> MVVNTIYIARHGYRSNWLPEGPYPDPLTGIDSDVPLAEHGVQQAKELAHYLLSLDNQPEAAFASPFYRCLETVQPIAKLLEIPVYLERGIGEWYRPDRKPVIPVPAGYEILSKFFPGVISQEWDSTLTPNEKGETEQEMYMRFKKFWPLFIERVEKEYPNVECILLVTHAASKIALGMSLLGYDNPRMSLNENGDKIRSGSCSLDKYEILKKSYDTIDETDDQTSFTYIPFSDRKWVLTMNGNTEFLSSGEEMNWNFDCVAEAGSDADIKKRQMTKKTSSPIPEADDQTEVETVYISVDIPSGNYKERTEIAKSAILQYSGLETDAPLFRIGNRLYEGSWERLVGTELAFPNAAHVHKK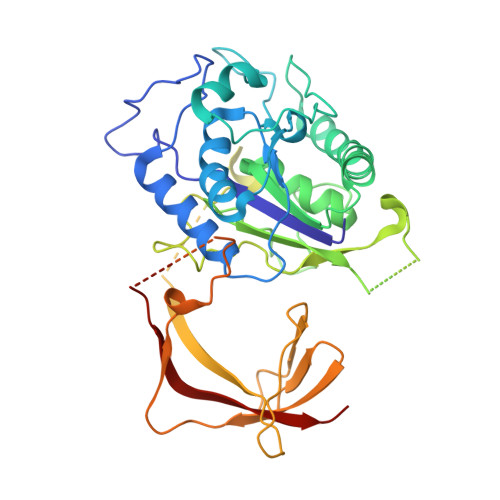TAGLLSPTEENETTNAGQSKGSSTANDPNIQIQEEDVGLPDSTNTSRDHTGDKEEVQSEKIYRIKERIVLSNVRPM N-[(3S)-3-{[(3S)-3-amino-3-carboxypropyl]amino}-3-carboxypropyl]-L-glutamic acid | C13 H23 N3 O8 | 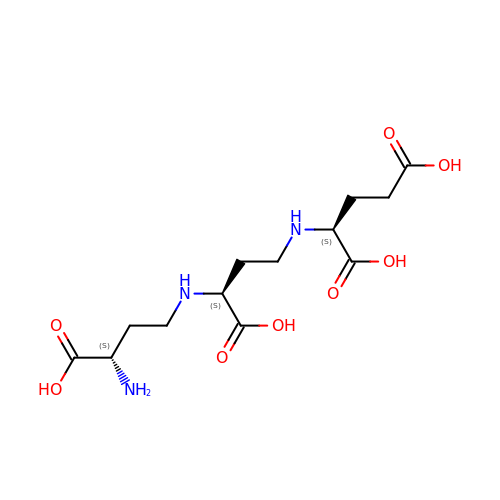PCXSNYIAEDAACL-CIUDSAMLSA-N> MANPYERGPNPTDALLEARSGPFSVSEENVSRFGADGFGGGTIYYPRENNTYGAVAISPGYTGTQASVAWLGERIASHGFVVITIDTNTTLDQPDSRARQLNAALDYMINDASSAVRSRIDSSRLAVMGHSMGGGGTLRLASQRPDLKAAIPLTPWHLNKNWSSVRVPTLIIGADLDTIAPVLTHARPFYNSLPTSISKAYLELDGATHFAPNIPNKIIGKYSVAWLKRFVDNDTRYTQFLCPGPR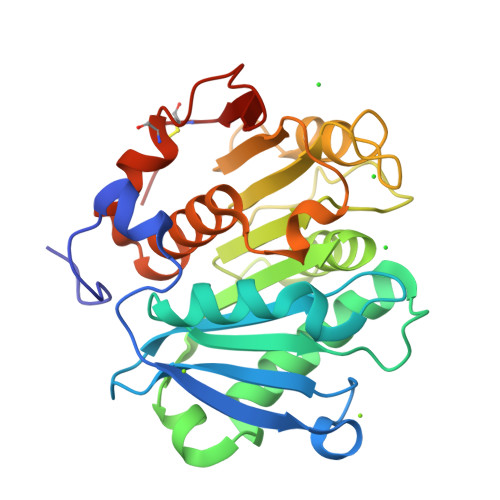DGLFGEVEEYRSTCPFALE> MFAIDPLKHPKLYEEYGLYLRPHQINQEIKPTTIKKKELAPTIRSIKYASLIHSMLAKHAARHNGTLINPRMYADMITLGNTKVTVTKGTPKAQIDTLKMNGLTVVSKSRRNNKKKPVSDTTASTDETTDDVVTYKALTEMSTLVESFRLPSGLTLIVFDDEKYQSLIPDYINQLITYTQPHIIPTWQGITDFSDTYLRSYFKRPFELTASNLAVPQKHNLSPITRSIFNNTGREDAIIRKLYGYGEYVFIKYEGCLITWTGLYGAVTMMVNLPKRDLGLDVGDDFLKEYKKLLFHGVITDAIPSGISAKSTVMRISPHKMMNPSGGALAVLSKYIEAVVSTNVINATLVVYAEKGAGKTSFLSTYAQQLSLASGQIVGHLSSDAYGRWLAKNKDVEEPSFEYDYVLSLDTDDNESYYEQKASELLTSHGISELSQYELLSVRRKVKMMNEMDEILIAQLDNANTHSERNFYYMVSTGKNTPRTLIVEGHFNAQDATIARTDTTILLRTINDTTQAMRDRQRSGVVQLFLRDTYYRLLPSLHTTVY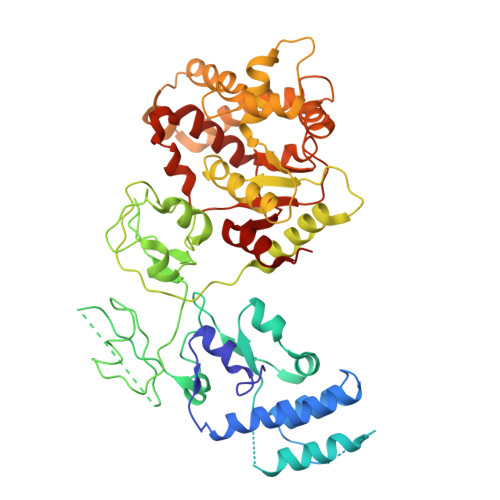PFEMLESIKRWKWVH(2~{R})-2-[4-(3-fluoranyl-4-methyl-phenyl)-3-(trifluoromethyl)phenyl]butanoic acid | C18 H16 F4 O2 | 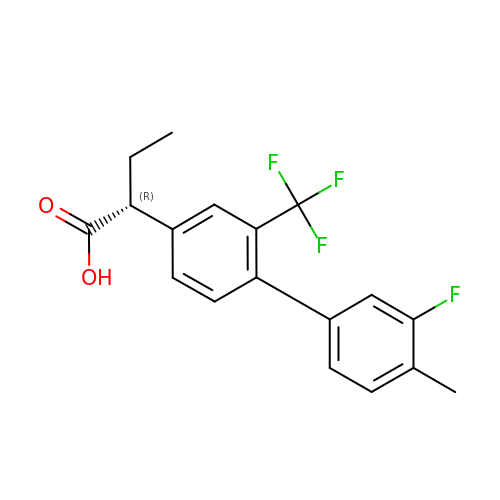IZMCUINTVDMYCG-CYBMUJFWSA-N>MVTFLEKISERAKKLNKTIALPETEDIRTLQAAAKILERGIADIVLVGNEADIKALAGDLDLSKAKIVDPKTYEKKDEYINAFYELRKHKGITLENAAEIMSDYVYFAVMMAKLGEVDGVVSGAAHSSSDTLRPAVQIVKTAKGAALASAFFIISVPD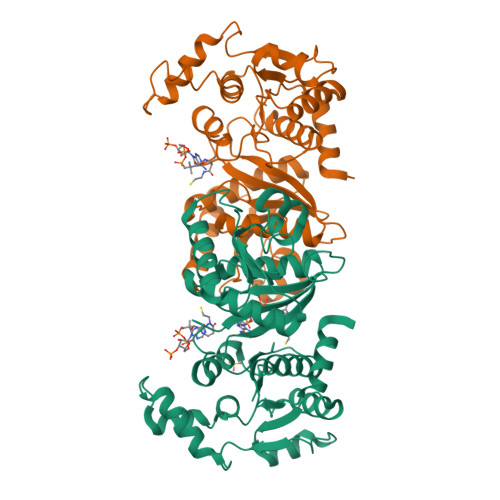CEYGSDGTFLFADSGMVEMPSVEDVANIAVISAKTFELLVQDVPKVAMLSYSTKGSAKSKLTEATIASTKLAQELAPDIAIDGELQVDAAIVPKVAASKAPGSPVAGKANVFIFPDLNCGNIAYKIAQRLAKAEAYGPITQGLAKPINDLSRGCSDEDIVGAVAITCVQAAAQDK[2x]Two of the main force transduction components are talin and vinculin. As forces increase in FAs, vinculin moves away from the membrane towards the force transduction and actin rich layers in a myosin II dependent manner. A direct interaction between FAK and vinculin is not reported, but both are shown to interact with the FA adaptor protein paxillin. Here we demonstrate that paxillin can act as an adaptor protein to connect FAK with the force transduction component vinculin.

We therefore set out to obtain structural information for LD2 binding to vinculin and performed crystallization experiments with Vin-T bound to LD2 and/or LD1 (the latter since we observed considerable affinity for LD1 to Vin-T). Interestingly, we only obtained crystals in presence of both, LD1 and LD2 peptides. Diffraction of optimized crystals resulted in a crystal structure at a resolution of 2.55 Å. In the final structure, the asymmetric unit contains four Vin-T molecules and each two LD1 and LD2 peptides, which are well defined in the electron density maps. Together, this assembly forms a circular arrangement that contains a non-crystallographic 2-fold symmetry. At 100 µM approximately 20% of Vin-T converts to a form sedimenting with ~ 2.5 S, compatible with dimeric Vin-T. Neither the presence of LD1, LD2 or both peptides significantly changed the sedimentation behavior of Vin-T, suggesting that the multimeric assembly seen in the crystal structure does not form in solution at concentrations up to 100 µM. There are three different Vin-T:LD interactions observed in the crystal structure, one involving LD1 and two LD2, each is present twice due to the non-crystallographic symmetry. Analysis with the PISA server indicates that the most energetically favorable and most specific interaction (with significant hydrophobic character) is observed between LD2 and the Vin-T chains B and D. This interaction involves the LD residues in LD2 and rigid residues within helices 2 and 3 (H2, H3) in Vin-T. We therefore conclude that of the Vin-T:LD interactions observed in the crystal structure, only the LD2 interaction with helices H2 and H3 in Vin-T is compatible with a simultaneous role of vinculin in force transduction.

>[4x]GPLGSGEVINQPMMMAARQLHDEARKWSSKGNDIIAAAKRMALLMAEMSRLVRGGSGTKRALIQCAKDIAKASDEVTRLAKEVAKQCTDKRIRTNLLQVCERIPTISTQLKILSTVKATMLGRTNISDEESEQATEMLVHNAQNLMQSVKETVREAEAASIKIRTDAGFTLRWVRKTPWYQ;>[2x]SNLSELDRLLLELNAVQHN;>[2x]MDDLDALLADLES>[2x]SNADSLPERIDLFVSLFDYNSATTSYDIRSIQTDFPTRLLTPDSMLPQTSEYPLKDIQLLYKLAQSCTGKLPLSPLITEPLVFTRSLCKGS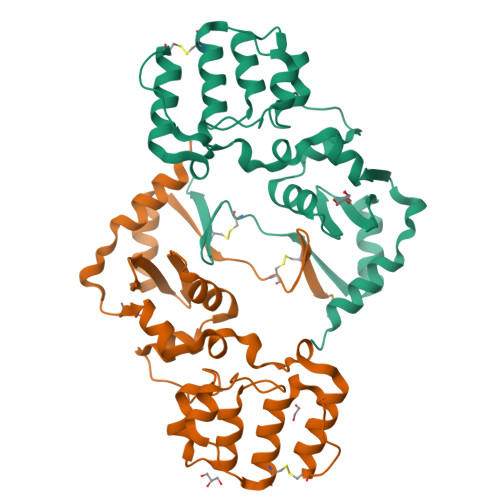SLSPRWFARSGLIHPGGGTYAFRYAEKYPAQFANLLPYMHIQERPNAAEGTLLYHLQNMGEDAINALVSGASMFGSGSDLWLRKGDIYYLFNEETWLTNANKAGLSYSLLSACFIQRGNICWDVEDHS>TYRVXTWE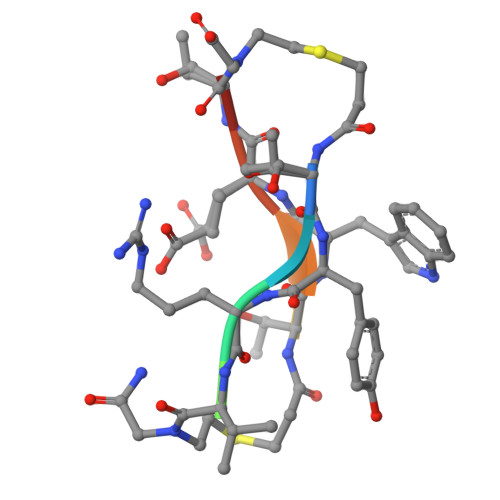TX[2x]>GCCGGC[2x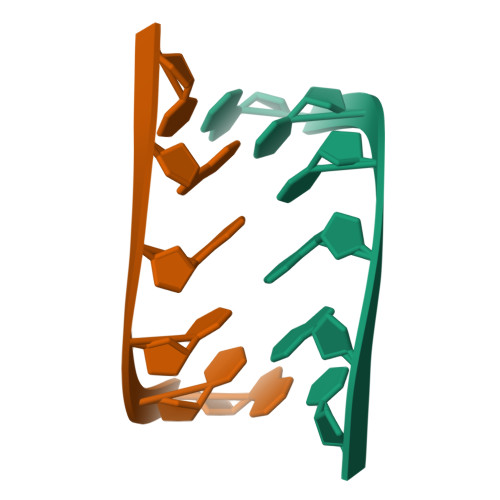]> GWSKVVNFLNKGVQRRPHRRLPGQPHHQWNMLKTQLDQLVRSDRLELTLPRAHELQQYAEELVHFAKQNTPESSLIVESMIFTPAARR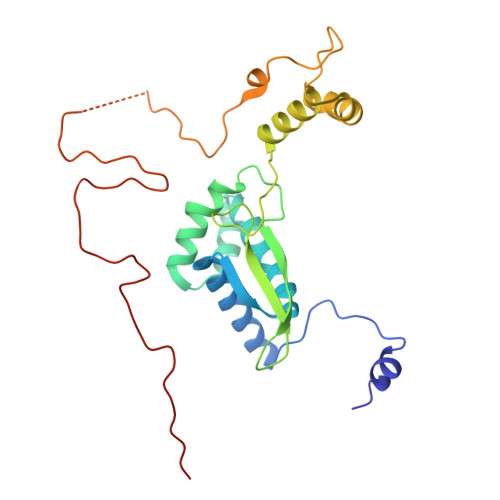KLFHELCPLYANRPFFYTRVVNQHRLRMRDAAPMAYLEFVDRPGEIRPARPVGFERKQAIWEEMQATRRGRRQWWNHAKKLGLIDEETGDVISDINALRRPSAAEWEESDSEEEKADSPSPYKMVAAPKRALEPFFVDLPPPTERYRKQRYVFKRFRP BUTYRAMIDE | C4 H9 N O | 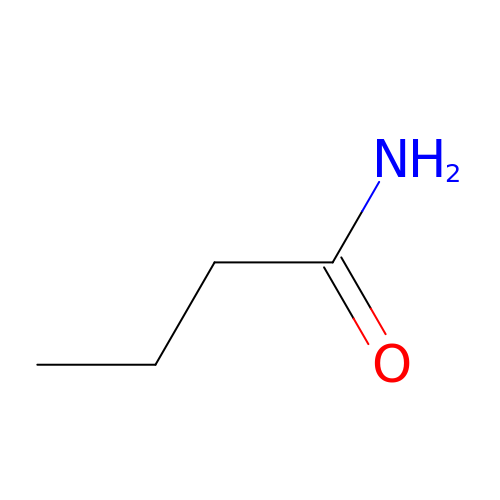DNSISZSEWVHGLH-UHFFFAOYSA-N4-({N-[2-(benzylamino)-2-oxoethyl]-4-(dimethylamino)benzamido}methyl)-3-fluoro-N-hydroxybenzamide | C26 H27 F N4 O4 | 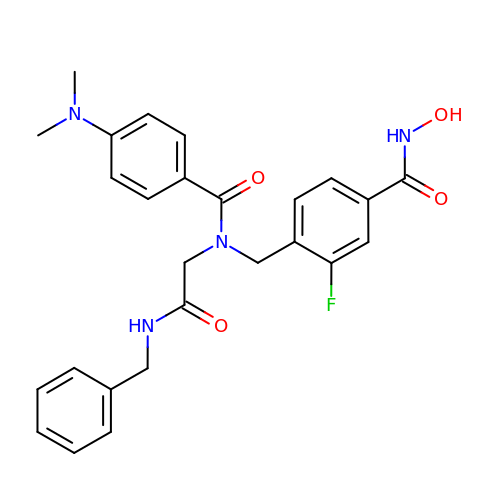GBIQEYYBFBGNOZ-UHFFFAOYSA-N>[2x]SMKDVPDSQQHPAPEKSSKVS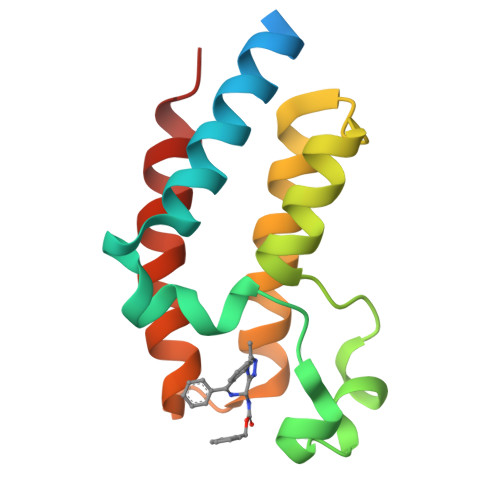EQLKCCSGILKEMFAKKHAAYAWPFYKPVDVEALGLHDYCDIIKHPMDMSTIKSKLEAREYRDAQEFGADVRLMFSNCYKYNPPDHEVVAMARKLQDVFEMRFAKMPDE3-(diethylamino)phenol | C10 H15 N O | 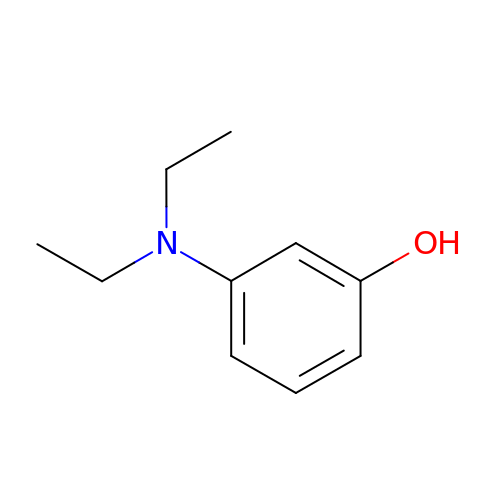WAVOOWVINKGEHS-UHFFFAOYSA-N> MALLAEHLLKPLPAD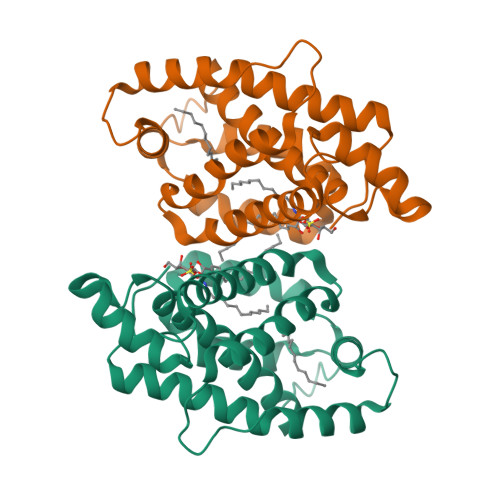KQIETGPFLEAVSHLPPFFDCLGSPVFTPIKAVISGNITKIKAVYDTNPAKFRTLQNILEVEKEMYGAEWPKVGATLALMWLKRGLRFIQVFLQSICDGERDENHPNLIRVNATKAYEMALKKYHGWIVQKIFQAALYAAPYKSDFLKALSKGQNVTEEECLEKIRLFLVNYTATIDVIYEMYTQMNAELNYKV>[2x]SHMGQGGSNPKFE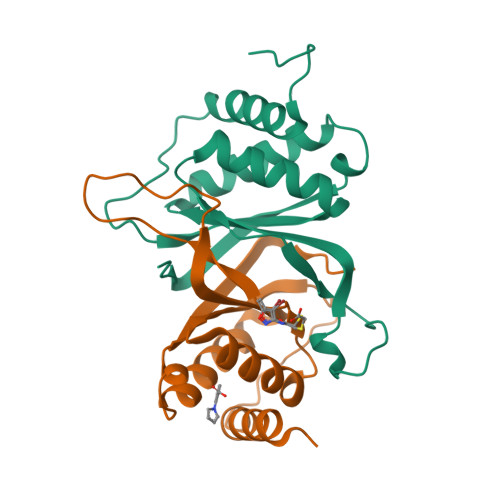NIAEGLRALLARSHVERTTDEGTWVAGVFVYGGSKTSLYNLRRGTALAIPQCRLTPLSRLPFGMAPGPGPQPGPLRESIVCYFMVFLQTHIFAEVLKDAIKDLVMTKPAPTCNIRVTVCSFDDGVDLP> GSHMLSDEQMQIINSLVEAHHKTYDDSYSDFVRFRPPVREGPVTRSASRAASLHSLSDASSDSFNHSPESVDTKLNFSNLLMMYQDSGSPDSSEEDQQSRLSMLPHLADLVSYSIQKVIGFAKMIPGFRDLTAEDQIALLKSSAIEIIMLRSNQSFSLEDMSWSCGGPDFKYCINDVTKAGHTLELLEPLVKFQVGLKKLKLHEEEHVLLMAICLLSPDRPGVQDHVRIEALQDRLCDVLQAYIRIQHPGGRLLYAKMI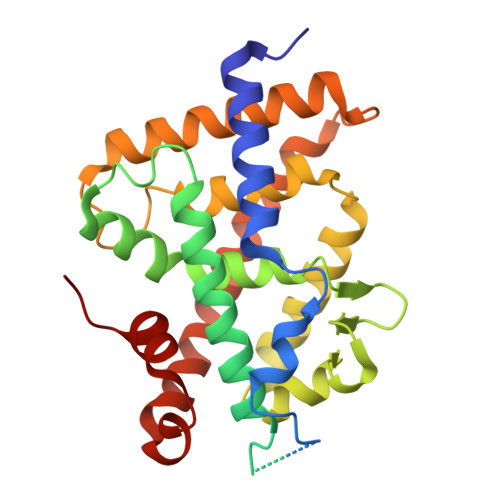QKLADLRSLNEEHSKQYRSLSFQPEHSMQLTPLVLEVFGSEVS>GLHALMTAEELAFFARFGRMREIAAGQALFERGAVGTQMFIVVTGQIDLDFGEDLMLKHLGPGEFFGELGLLIGDHARSAGASASVDSRLIELAHDDFQRLVDHDPSMVAHFLRRSIVRVVNNEQLL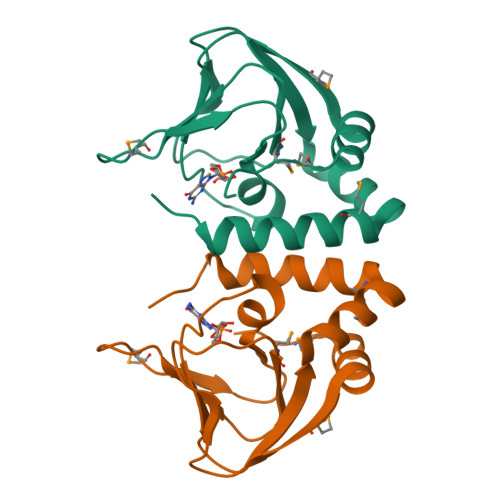IR[2x]>GPGSMPSERTFIAVKPDGVQRNLVGEIIKRFENKGYKL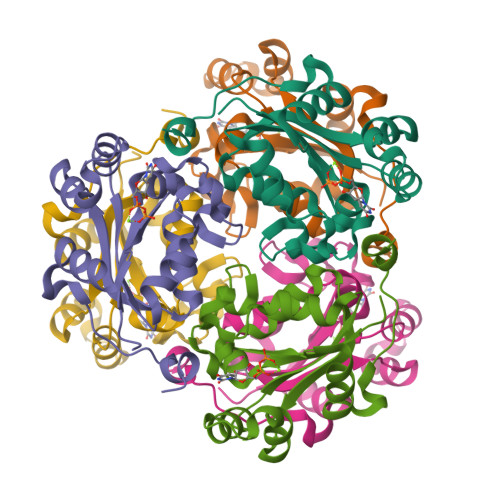VGLKLLQPTEEQAKQHYIDLASKPFYSGLVSYFSSGPIVGMVWEGLGVVKGGRVLLGATNPADSLPGTIRGDFAVDVGRNVCHGSDSVESAKREIAFWFKAEELVSWTSHSVKQIYERA[3x]>GMSTQYWEEEIEIMSREKLQELQLQRLKKTINIAANSPYYKEVFSKNGITGDSIQSLDDIRKIPFTTKSDMRANYPFGLVAGDMKRDGVRIHSSSGTTGNPTVIVHSQHDLDSWANLVARCLYMVGIRKTDVFQNSSGYGMFTGGLGFQYGAERLGCLTVPAAAGNSKRQIKFISDFKTTALHAIPSYAIRLAEVFQEEGIDPRETTLKTLVIGAEPHTDEQRRKIERMLNVKAYNSFGMTEMNGPGVAFECQEQNGMHFWEDCYLVEIIDPETGEPVPEGEIGELVLTTLDREMMPLIRYRTRDLTRILPGKCPCGRTHLRIDRIKGRSDDMFIIKGVNIFPMQVEKILVQFPELGSNYLITLETVNNQDEMIVEVELSDLSTDNYIELEKIRRDIIRQLKDEILVTPKVKLVKKGSLPQSE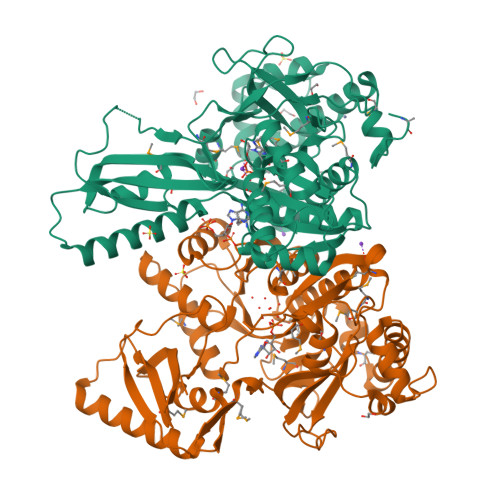GKAVRVKDLRDNK[4x]> STLEVRSQATQDLSEYYNRPYFDLRNLSGYREGNTVTFINHYQQTDVKLEGKDKDKIKDGNNENLDVFVVREGSGRQADNNSIGGITKTNRTQHIDTVQNVNLLVSKSTGQHTTSVTSTNYSIYKEEISLKELDFKLRKHL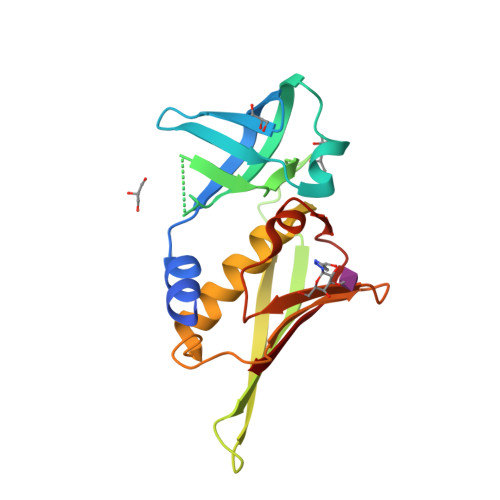IDKHDLYKTEPKDSKIRVTMKNGDFYTFELNKKLQTHRMGDVIDGRNIEKIEVNL> MKFAEHLSAHITPEWRKQYIQYEAFKDMLYSAQDQAPSVEVTDEDTVKRYFAKFEEKFFQTCEKELAKINTFYSEKLAEAQRRFATLQNELQSSLDAQKESTGVTTLRQRRKPVFHLSHEERVQHRNIKDLKLAFSEFYLSLILLQNYQNLNFTGFRKILKKHDKILETSRGADWRVAHVEVAPFYTCKKINQLISETEAVVTNELEDGDRQKAMKRLRVPPLGAAQPAPAWTTFRVGLFCGIFIVLNITLVLAAVFKLETDRSIWPLIRIYRGGFLLIEFLFLLGINTYGWRQAGVNHVLIFELNPRSNLSHQHLFEIAGFLGILWCLSLLACFFAPISVIPTYVYPLALYGFMVFFLINPTKTFYYKSRFWLLKLLFRVFTAPFHKVGFADFWLADQLNSLSVILMDLEYMICFYSLELKWDESKGLLPNNSEESGICHKYTYGVRAIVQCIPAWL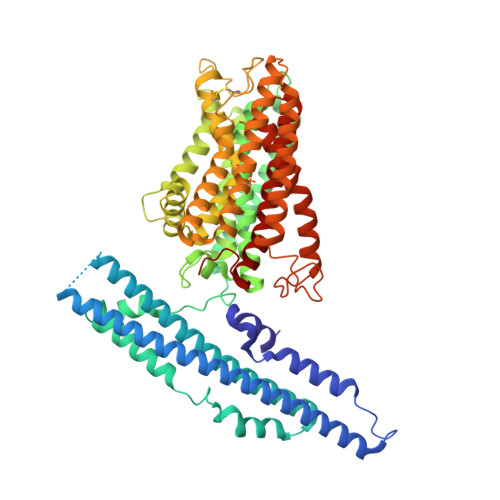RFIQCLRRYRDTKRAFPHLVNAGKYSTTFFMVTFAALYSTHKERGHSDTMVFFYLWIVFYIISSCYTLIWDLKMDWGLFDKNAGENTFLREEIVYPQKAYYYCAIIEDVILRFAWTIQISITSTTLLPHSGDIIATVFAPLEVFRRFVWNFFRLENEHLNNCGEFR> QDLTVKMTDLQTGKPVGTIELSQNKYGVVFIPELADLTPGEHGFHIHQNGSCASSEKDGKVVLGGAAGGHYDPEHTNKHGFPWTDDNHKGDLPALFVSANGLATNPVLAPRLTLKE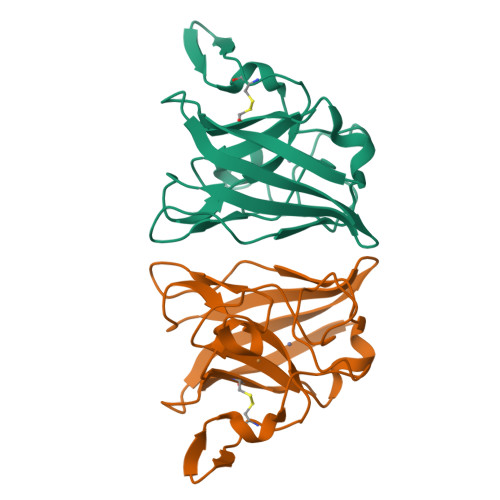LKGHAIMIHAGGDNHSDMPKALGGGGARVACGVIQ>[4x]MSLTYINKEKVIKNLSYAIYLLKKMNFTLIPEVGSNIAESLPFPKDFKDVAALTGRIIKN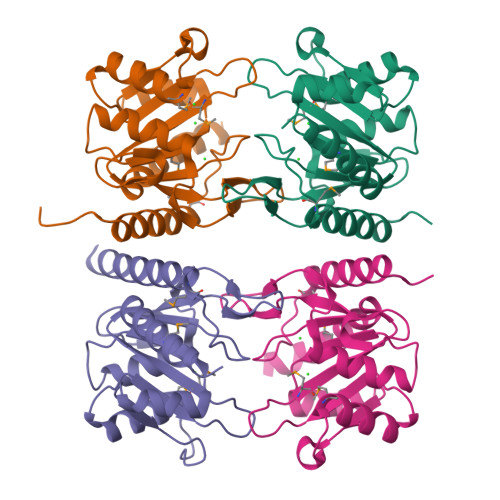KLGGFYIVGDIEFGASEHIAKIILSASKFNPEIRACMNIKYDGGLIKLLKDKFAVSSFDRKEEPPNVSTMEWGTKIACEKFGGVPDIIYDRGGEGKEPMIRVLGRDAIEVVKKVEVIQKIYNTLEGHHHHHH>MVIQWYPGHMAKAKREVSEQLKKVDVVFELVDARIPYSSRNPMIDEV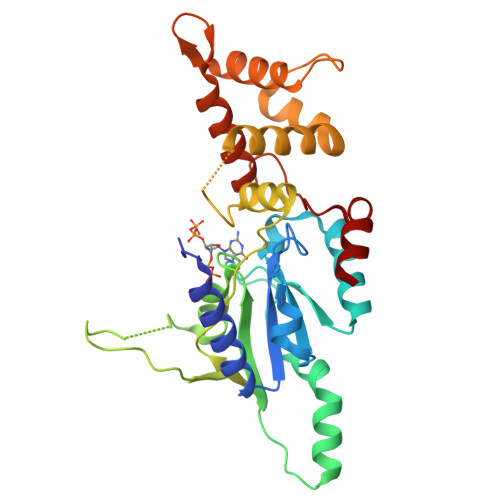INQKPRVVILNKKDMSNLNEMSKWEQFFIDKGYYPVSVDAKHGKNLKKVEAAAIKATAEKFEREKAKGLKPRAIRAMIVGIPNVGKSTLINKLAKRSIAQTGNKPGVTKQQQWIKVGNALQLLDTPGILWPKFEDEEVGKKLSLTGAIKDSIVHLDEVAIYGLNFLIQNDLARLKSHYNIEVPEDAEIIAWFDAIGKKRGLIRRGNEIDYEAVIELIIYDIRNAKIGNYCFDIFKDMTEELANDANN[2x]>MSLKIAVTGGTGFLGQYVVESIKNDGNTPIILTRSIGNKAINDYEYRVSDYTLEDLINQLNDVDAVVHLAATRGSQGKISEFHDNEILTQNLYDACYENNISNIVYASTISAYSDETSLPWNEKELPLPDLMYGVSKLACEHIGNIYSRKKGLCIKNLRFAHLYGFNEKNNYMINRFFRQAFHGEQLTLHANSVAKREFLYAKDAAKSVIYA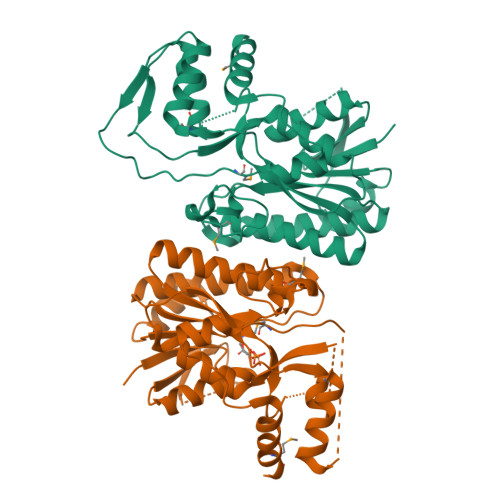LKQEKVSGTFNIGSGDALTNYEVANTINNAFGNKDNLLVKNPNANEGIHSSYMDSSKAKELLDFSTDYNFATAVEEIHLLMRGLDDVPLWYEGHHHHHH[6x]>[2x]MGHRIPEETIEAIRRGVDIVDVIGEY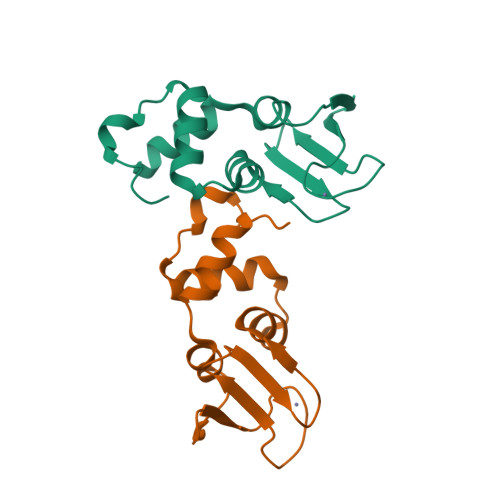VQLKRQGRNYFGLCPFHGEKTPSFSVSPEKQIFHCFGCGAGGNAFTFLMDIEGIPFVEAAKRLAAKAGVDLSVYELD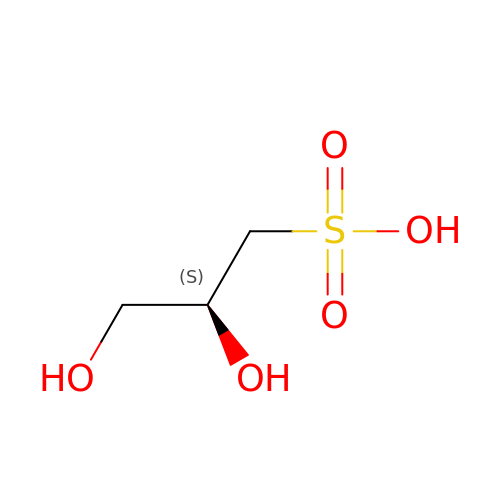(2~{S})-2,3-bis(oxidanyl)propane-1-sulfonic acid | C3 H8 O5 S | YPFUJZAAZJXMIP-VKHMYHEASA-N N-(2-isopropoxy-3-(4-methylpiperazine-1-carbonyl)phenyl)-4-oxo-3,4-dihydrothieno[3,2-d]pyrimidine-7-carboxamide | C22 H25 N5 O4 S | 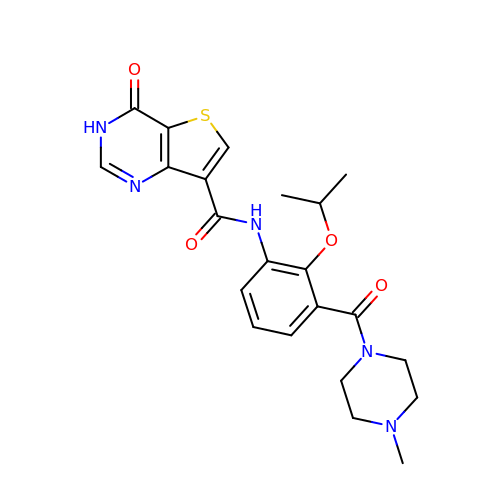MJJJFOLDERHCND-UHFFFAOYSA-N3,5-dimethyl-4-{[2-({1-[4-(methylsulfonyl)benzyl]piperidin-4-yl}amino)pyrimidin-4-yl]oxy}benzonitrile 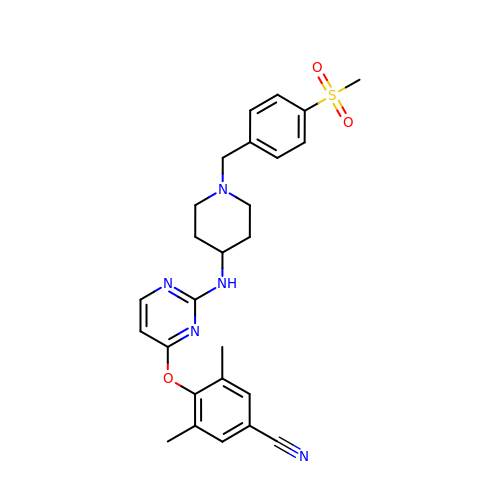| C26 H29 N5 O3 S | LPBHCIIMBZNWQE-UHFFFAOYSA-N> MDYKDDDDKGDHNHRHKHGDPLEVLFQGPGGDPHMSRESNDTIQSDTVRSSSKSDYFRIQLNNQDYYMSKPTFLDPSHGESLPLNQFSQVPNIRVFGALPTGHQVLCHVHGILPYMFIKYDGQITDTSTLRHQRCAQVHKTLEVKIRASFKRKKDDKHDLAGDKLGNLNFVADVSVVKGIPFYGYHVGWNLFYKISLLNPSCLSRISELIRDGKIFGKKFEIYESHIPYLLQWTADFNLFGCSWINVDRCYFRSPV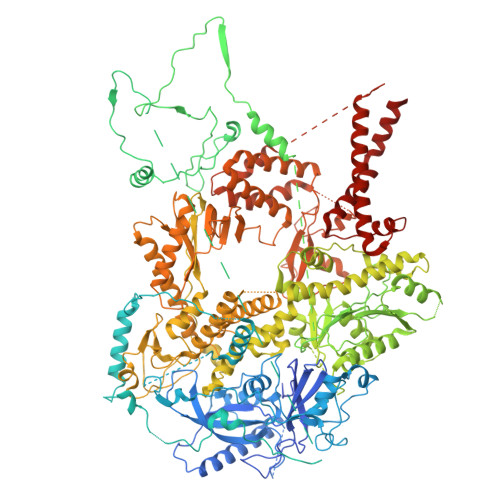LNSILDIDKLTINDDLQLLLDRFCDFKCNVLSRRDFPRVGNGLIEIDILPQFIKNREKLQHRDIHHDFLEKLGDISDIPVKPYVSSARDMINELTMQREELSLKEYKEPPETKRHVSGHQWQSSGEFEAFYKKAQHKTSTFDGQIPNFENFIDKNQKFSAINTPYEALPQLWPRLPQIEINNNSMQDKKNDDQVNASFTEYEICGVDNENEGVKGSNIKSRSYSWLPESIASPKDSTILLDHQTKYHNTINFSMDCAMTQNMASKRKLRSSVSANKTSLLSRKRKKVMAAGLRYGKRAFVYGEPPFGYQDILNKLEDEGFPKIDYKDPFFSNPVDLENKPYAYAGKRFEISSTHVSTRIPVQFGGETVSVYNKPTFDMFSSWKYALKPPTYDAVQKWYNKVPSMGNKKTESQISMHTPHSKFLYKFASDVSGKQKRKKSSVHDSLTHLTLEIHANTRSDKIPDPAIDEVSMIIWCLEEETFPLDLDIAYEGIMIVHKASEDSTFPTKIQHCINEIPVMFYESEFEMFEALTDLVLLLDPDILSGFEIHNFSWGYIIERCQKIHQFDIVRELARVKCQIKTKLSDTWGYAHSSGIMITGRHMINIWRALRSDVNLTQYTIESAAFNILHKRLPHFSFESLTNMWNAKKSTTELKTVLNYWLSRAQINIQLLRKQDYIARNIEQARLIGIDFHSVYYRGSQFKVESFLIRICKSESFILLSPGKKDVRKQKALECVPLVMEPESAFYKSPLIVLDFQSLYPSIMIGYNYCYSTMIGRVREINLTENNLGVSKFSLPRNILALLKNDVTIAPNGVVYAKTSVRKSTLSKMLTDILDVRVMIKKTMNEIGDDNTTLKRLLNNKQLALKLLANVTYGYTSASFSGRMPCSDLADSIVQTGRETLEKAIDIIEKDETWNAKVVYGDTDSLFVYLPGKTAIEAFSIGHAMAERVTQNNPKPIFLKFEKVYHPSILISKKRYVGFSYESPSQTLPIFDAKGIETVRRDGIPAQQKIIEKCIRLLFQTKDLSKIKKYLQNEFFKIQIGKVSAQDFCFAKEVKLGAYKSEKTAPAGAVVVKRRINEDHRAEPQYKERIPYLVVKGKQGQLLRERCVSPEEFLEGENLELDSEYYINKILIPPLDRLFNLIGINVGNWAQEIVKSKRASTTTTKVENITRVGTSATCCNCGEELTKICSLQLCDDCLEKRSTTTLSFLIKKLKRQKEYQTLKTVCRTCSYRYTSDAGIENDHIASKCNSYDCPVFYSRVKAERYLRDNQSVQREEALISLNDW>[2x]SNAMKKKILATLLTGLVLGTSLVGCGKTEGAEAGKKLVVSTWGLNEDVLKETVFEPFAKEHGVEIVLDIGNNSERLTKMKNNPNSQIDITYLAESFAEQGVEAGIFDKLDYSKIPNASEMNEKAKSTVEAGYGPAYTLNSIGIVVDPSAGIEINSWEDLWKPELKNKIAIPDITTTNGPAMVEIAAEKAGVDVKTDNGEAAFKE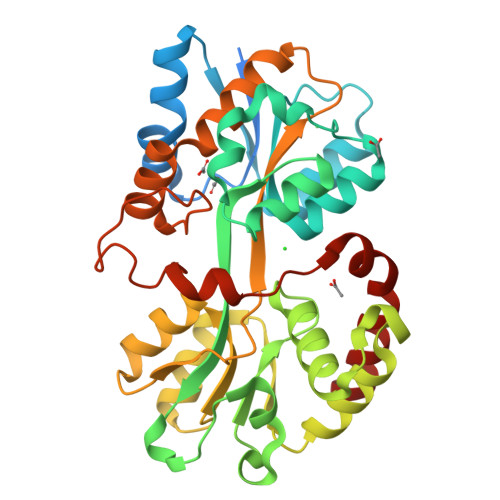LEALKPNVVKTYSKSSDLANMFSNGEIVAAVASDFAFGTISKAKPEVINVIPESGTYLNFNTININKNSKNKDLAYEFINYALSKEVQEKTAKALNESPVNKEVKLSEEETKNLTYGPVVDNAKVIDFKFVNSVMDQWVNNWNRIMN> NIVHNYSEAEIKVREATSNDPWGPSSSLMSEIADLTYNVVAFSEIMSMIWKRLNDHGKNWRHVYKAMTLMEYLIKTGSERVSQQCKENMYAVQTLKDFQYVDRD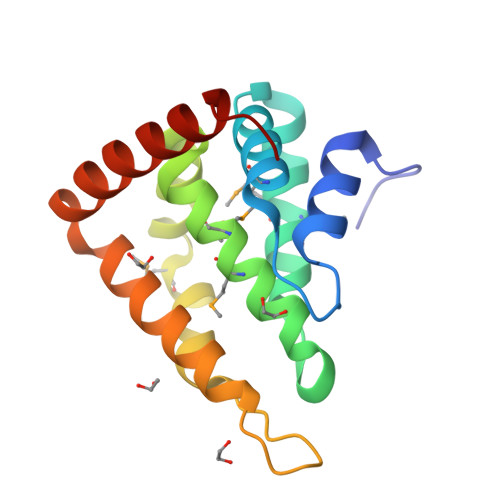GKDQGVNVREKAKQLVALLRDEDRLREERAHALKTKEKLAQTATA>MSQAIGILELTSIAAGMELGDAMLKSANVDLLVSKTISPGKFLLMLGGDIGAIQQAIETGTSQAGELLVDSLVLANIHPSVLPAISGLNSVDKRQAVGIVETWSVAACISAADRAVKGSNVTLVRVHMAFGIGGKCYMVVAGDVSDVALAVT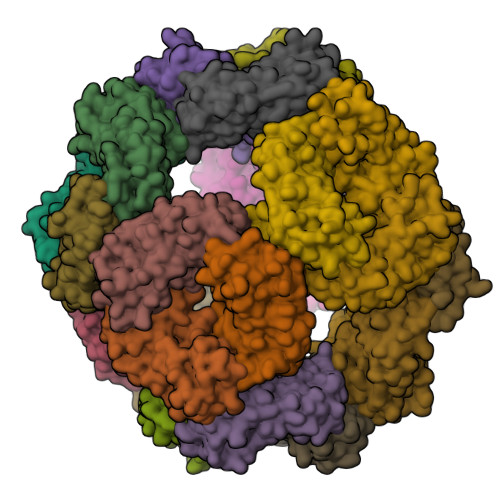VASSSAGAYGLLVYASLIPRPHEAMWRQMVEGLEHHHHHH[8x]>[4x]GSHMGEGEGVQLTAAQELMIQQLVAAQLQCNKRSFSDQPKVTPWPLGADPQSRDARQQRFAHFTELAIISVQEIVDFAKQVPGFLQLGREDQIALLKASTIEIMLLETARRYNHETECITFLKDFTYSKDDFHRAGLQVEFINPIFEFSRAMRRLGLDDAEYALLIAINIFSADRPNVQEPG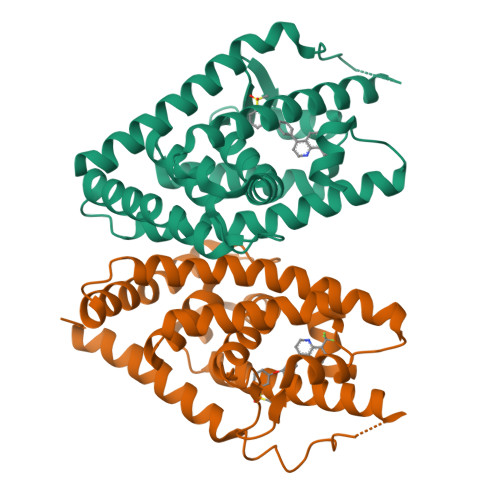RVEALQQPYVEALLSYTRIKRPQDQLRFPRMLMKLVSLRTLSSVHSEQVFALRLQDKKLPPLLSEIWDVHE>AGGHGDVGMHVKEKEKNKDENKRKDEERNKTQEEHLKEIMKHIVKIEVKGEEAVKKEAAEKLLEKVPSDVLEMYKAIGGKIYIVDGDITKHISLEALSEDKKKIKDIYGKDALLHEHYVYAKEGYEPVLVIQSSEDYVENTEKALNVYYEIGKILSRDILSKINQPYQKFLDVLNTIKNASDSDGQDLLFTNQLKEHPTDFSVEFLEQNSNEVQEVFAKAFAYYIEPQHRDVLQLYAPEAFNYMDKFNEQEINLSLEELKDQRMLSRYEKWEKIKQHYQHWSDSLSEEGRGLLKKLQIPIEPKKDDIIHSLSQEEKELLKRIQIDSSDFLSTEEKEFLKKLQIDIRDSLSEEEKELLNRIQVDSSNPLSEKEKEFLKKLKLDIQPYDINQRLQDTGGLIDSPSINLDVRKQYKRDIQNIDALLHQSIGSTLYNKIYLYENMNINNLTATLGADLVDSTDNTKINRGIFNEFKKNFKYSISSNYMIVDINERPALDNERLKWRIQLSPDTRAGYLENGKLILQRNIGLEIKDVQIIKQSEKEYIRIDAKVVPKSKIDTKIQEAQLNINQEWNKALGLPKYTKLITFNVHNRYASNIVESAYLILNEWKNNIQSDLIKKVTNYLVD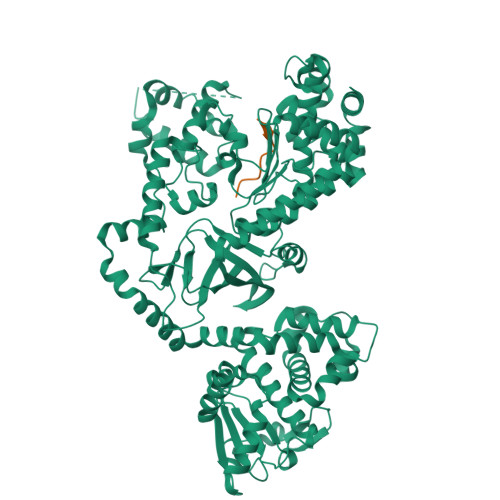GNGRFVFTDITLPNIAEQYTHQDEIYEQVHSKGLYVPESRSILLHGPSKGVELRNDSEGFIHEFGHAVDDYAGYLLDKNQSDLVTNSKKFIDIFKEEGSNLTSYGRTNEAEFFAEAFRLMHSTDHAERLKVQKNAPKTFQFINDQIKFIINS[2x];>MLARRKKVYPYPMEPTIAEG[2x]> MVSVIKPEMKMRYYMDGSVNGHEFTIEGEGTGRPYEGHQEMTLRVTMAKGGPMPFAFDLVSHVFCYGHRPFTKYPEEIPDYFKQAFPEGLSWERSLEFEDGGSASVSAHISLRGNTFYHKSKFTGVNFPADGPIMQNQSVDWEPSTEKITASDGVLKGDVTMYLKLEGGGNHKCQFKTTYKAAKKILKMPGSHYISHRLVRKTEGNITELVEDAVAHSLEHH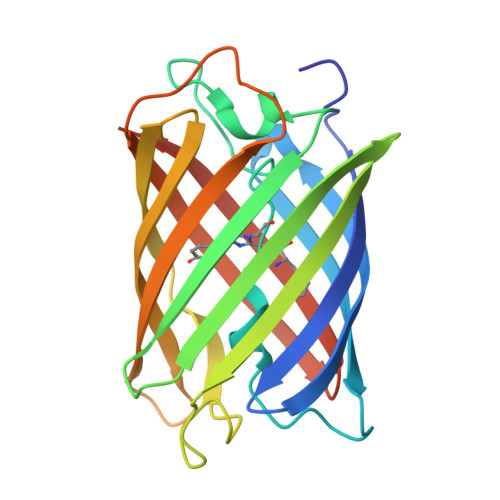HHHH>[2x]MAADIFAKFKKSMEVKFTQEYGSNKQAGGDITGKTEKFLRLGPEQDARKQEMIKAGKEIAEKRGIAFYNPMMHMGAPLGQRAITPYTISGTDIVAEPDDLHYVNNAAMQQMWDDIRRTCIVGLDMAHETLEKRLGKEVTPETINHYLETLNHAMPGAAVVQEMMVETHPALVDDCYVKIFTGDDELADEIDKQYVINVNKMFSEEQAAQIKASIGKTTWQAIHIPTIVSRTTDGAQTSRWAAMQIGMSFISAYAMCAGEAAVADLSFAAKHAALVSMGEMLPARRARGPNEPGGLSFGHLSDIVQTSRVSKDPAKIALEVVGAGCMLYDQIWLGSYMSGGVGFTQYATAAYTDDILDNNTYYDVDYINDKYNGAANLGTDNKVKATLDVVKDIATESTLYGIETYEKFPTALEDHFGGSQRATVLAAASGVACALATGNANAGLSGWYLSMYVHKEAWGRLGFFGFDLQDQCGATNVLSYQGDEGLPDELRGPNYPNYAMNVGHQGGYAGIAQAAHSGRGDAFTVNPLLKVCFADELMPFNFAEPRREFGRGAIREFMPAGERSLVIPAK;>[2x]MSDTVDIYDDRGKLLESNVDIMSLAPTRNAAIKKIILDTKRSVAVSLAGIQGALASGKMGGKGRQILGRGLNYDLVGNADAIAENVKNLVQVDEGDDTSVKVIKGGKSLLIQAPSSRIAAGADYMSATTVGAAAVTQTIIDMFGTDMYDAPIAKSAVWGSYPQTMDLMGGNVQGVLSIPQNNEGLGFSLRNIMANHIAAITSRGAMNAAALSSIYEQSGIFEMGGAVGMFERHQLLGLACQGLNANNVVYDIVKENGKDGTIGTVIESIVGRAVEDGVISVDKTAPSGYKFYKANDVPMWNAYAAAGTLAATFVNCGAGRAAQNVSSTLLYFNDILEKETGLPGCDYGKVQGVAVGFSFFSHSIYGGGGPGVFNGNHVVTRHSRGFAIPCVCAAVALDAGTQMFTIESTSGLIGDVFGSIEEFRQPIK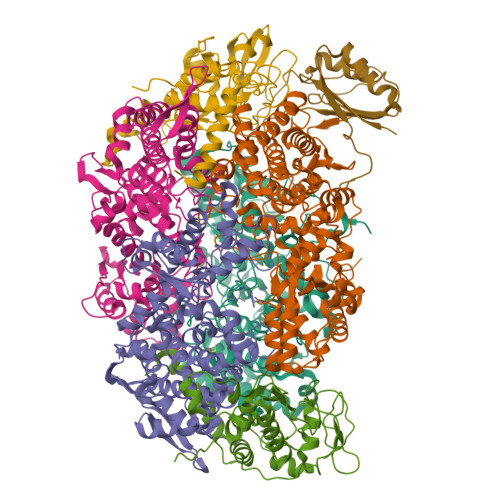AVAGAL;>[2x]MAYEAQYYPGATSVGANRRKHMSGKLEKLREISDEDLTAVLGHRAPGSDYPSTHPPLAEMGEPACSIREAVAATPGAAAGDRVRYVQFADSMYNAPATPYFRSYFAAINFRGVDPGTLSGRQIVEARERDMEQCAKVQMETEMTDPALAGMRGATVHGHSVRLQEDGVMFDMLDRRRLEGGVIIMDKDQVAIPLDRKVNLGKPMSSEEAAKRTTIYRVDNVAFRDDAEVIEWVHRVFDQRTSYGFQPK;> MDYKDDDDKGGGWSHPQFEKGGGMSDSASNTEDSIQIEIFPSRILSPETAQKLISELYQVDGIIRVMVQGPRLPERVSAGPGTGEKVEHPLRKPIQIGDQVIELKISVGRIRLEIENAETKEKVRSVCDKMLPFSFEFREGHFLRRKPTVTDYAKLGPETDPRLLGMVDPKAKVNQLVFIEKREKEDDTDKDE> PISPIETVPVKLKPGMDGPKVKQWPLTEEKIKALVEICTEMEKEGKISKIGPENPYNTPVFAIKKKDSTKWRKLVDFRELNKRTQDFWEVQLGIPHPAGLKKNKSVTVLDVGDAYFSVPLDEDFRKYTAFTIPSINNETPGIRYQYNVLPQGWKGSPAIFQSSMTKILEPFKKQNPDIVIYQYMDDLYVGSDLEIGQHRTKIEELRQHLLRWGLTTPDKKHQKEPPFLWMGYELHPDKWTVQPIVLPEKDSWTVNDIQKLVGKLNWASQIYPGIKVRQLSKLLRGTKALTEVIPLTEEAELELAENREILKEPVHGVYYDPSKDLIAEIQ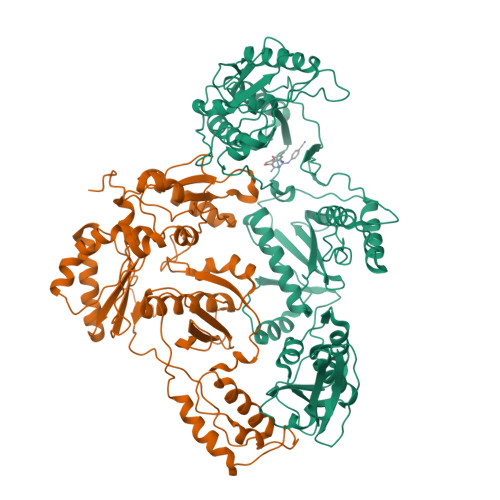KQGQGQWTYQIYQEPFKNLKTGKYARMRGAHTNDVKQLTEAVQKITTESIVIWGKTPKFKLPIQKETWETWWTEYWQATWIPEWEFVNTPPLVKLWYQLEKEPIVGAETFYVDGAANRETKLGKAGYVTNKGRQKVVPLTNTTNQKTELQAIYLALQDSGLEVNIVTDSQYALGIIQAQPDKSESELVNQIIEQLIKKEKVYLAWVPAHKGIGGNEQVDKLVSAGIRKIL;> PISPIETVPVKLKPGMDGPKVKQWPLTEEKIKALVEICTEMEKEGKISKIGPENPYNTPVFAIKKKDSTKWRKLVDFRELNKRTQDFWEVQLGIPHPAGLKKNKSVTVLDVGDAYFSVPLDEDFRKYTAFTIPSINNETPGIRYQYNVLPQGWKGSPAIFQSSMTKILEPFKKQNPDIVIYQYMDDLYVGSDLEIGQHRTKIEELRQHLLRWGLTTPDKKHQKEPPFLWMGYELHPDKWTVQPIVLPEKDSWTVNDIQKLVGKLNWASQIYPGIKVRQLSKLLRGTKALTEVIPLTEEAELELAENREILKEPVHGVYYDPSKDLIAEIQKQGQGQWTYQIYQEPFKNLKTGKYARMRGAHTNDVKQLTEAVQKITTESIVIWGKTPKFKLPIQKETWETWWTEYWQATWIPEWEFVNTPPLVKLWYQLE> GYFGKLESKLSVIRNLNDQVLFIDQGNRPLFEDMTDSDSRDNAPRTIFIISMYKDSQPRGMAVTISVKSEKISTLSSENKIISFKEMNPPDNIKDTKSDIIFFQRSVPGHDNKMQFESSSYEGYFLAS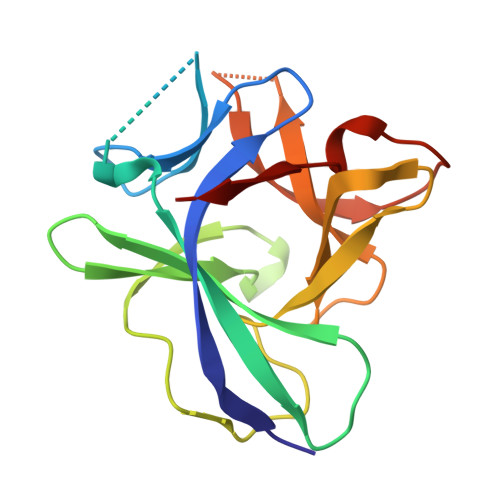EKERDLFKLILKKEDELGDRSIMFTVQNED>[2x]GSGSGMDEIVKVLSQHDRILVVGHIMPDGDCVSSVLSLTLGLEKLGKEVKAAVDYKIPYVFEKFPYIDKIEENPNFDPELLVVVDASSPDRIGKFQDLLDKVPSVVIDHHSTNTNFGNWNWVDPSFAATAQMIFRINKALGVEYDSNLATLNYLGIATDTGFFRHSNADVRVFEDAYKLVKMGADAHFVAKEILENK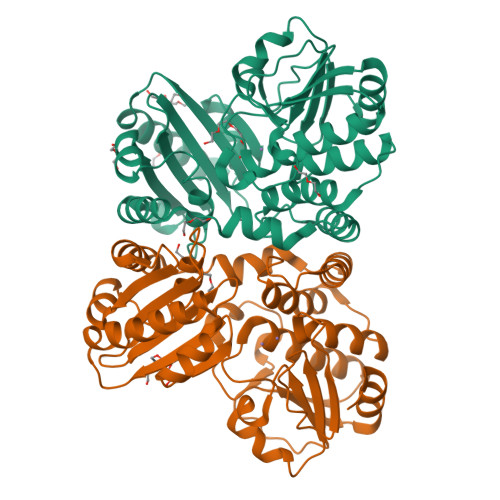RFEQFKLFAEVLERLQLLENGKIAYSYIDYDTYLRHNCTDEDSAGFVGELRSIRGVEVAVLFMEFPRGKIHVSMRSKDWFNVNEVAFELGGGGHPRAAGVTFEGKKIEEVIPRVINHLLKKFKEGVESESEKIPEGDVLGG>MPITLYSVSDGPPSLAVRQALEYLGLEHKLVNVDFGIGEHMTEEFAQKNPQKEIPVLDDNGFLLGESNAILQYLAERYGKDDTIYPKDPMARAVVNHRLCFNLSTYYRYISEYTLAPMFFDYQRTPLGLKKTHIALDNFNTYLKLLGKKYAAGETVTIADFQLVTATMCLEAINFDISPWPLVENWYDTYKLEHPTLWKIVEGGMKELEAFEKNPPDLSHMDHPIHPVRK[2x]

Glutathione S-transferases (GSTs) constitute a large superfamily of multifunctional enzymes that are ubiquitously present in both prokaryotes and eukaryotes. In general, GSTs catalyze the conjugation of the reduced glutathione (GSH)—a nucleophilic tripeptide comprised of three amino acids: cysteine, glutamic acid, and glycine—to a wide range of substrates that have an electrophilic carbon, nitrogen, or sulfur atom. In the current study, we identified an unclassified GST gene, LdGSTu1 from the Colorado potato beetle (CPB, Leptinotarsa decemlineata [Say]) in Coleoptera, which represents the most species-rich eukaryotic order, containing about half of the described herbivorous insect species (>400,000). The enzyme kinetic parameters and enzyme-substrate interaction studies demonstrated that LdGSTu1 could catalyze the conjugation of GSH to both CDNB and PNA, with a higher turnover number for CDNB than PNA.

Here, we solved the LdGSTu1 co-crystal structure with its nucleophilic substrate GSH by using X-ray diffraction. The LdGSTu1 structure was refined to a resolution of 1.80 Å. Two monomers of LdGSTu1 were in the crystal asymmetric unit. Chain A complexed with GSH has an open active site similar to previously published GST structures, whereas the chain B monomer vacant of GSH has a more closed active site, suggesting flexibility in loop-helix-loop region in the active site of the N-term domain of GSTs. The dimer is a result of crystal packing and not expected to be a biologically relevant dimer assembly as the active sites are solvent exposed and not internal to the dimer interface as reported for biological dimer assemblies in previous GST crystal structure studies. LdGSTu1 consists of two domains, the N-term domain and the C-term domain connected by a linker region coil. A molecular lipophilicity potential surface reveals that the LdGSTu1 substrate binding pocket has a more hydrophilic region on the N-term domain side of the binding pocket, which is bound with GSH and makes up the “G-site”, and a more lipophilic region in the substrate binding pocket adjacent to the bound GSH on the C-term domain side of the pocket making up the “H-site”. The GSH is bound to LdGSTu1 via an extensive hydrogen bonding network that includes amino acid side chains, backbone carbonyls, backbone amides and crystallographic water. The presumptive catalytic Ser14 formed a hydrogen bond with the thiol group of GSH bridged via a water molecule. The “H-site” of LdGSTu1 is largely hydrophobic and consists of Tyr107, Ser111, Leu115, Ala116, Phe119, Phe120, Leu208, Ala210, and Phe211.> HHAADYVLYKDATKPVEDRVADLLGRMTLAEKIGQMTQIERLVATPDVLRDNFIGSLLSGGGSV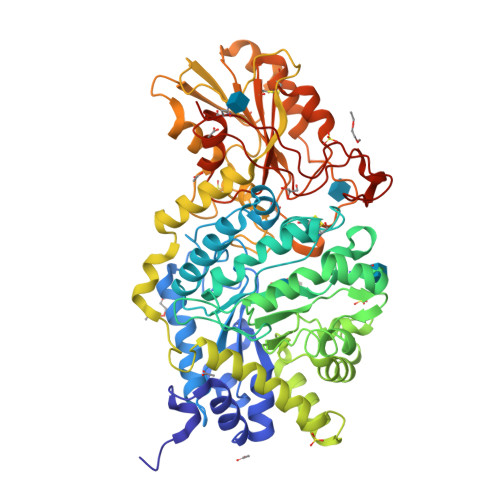PRKGATAKEWQDMVDGFQKACMSTRLGIPMIYGIDAVHGQNNVYGATIFPHNVGLGATRDPYLVKRIGEATALEVRATGIQYAFAPCIAVCRDPRWGRCYESYSEDRRIVQSMTELIPGLQGDVPKDFTSGMPFVAGKNKVAACAKHFVGDGGTVDGINENNTIINREGLMNIHMPAYKNAMDKGVSTVMISYSSWNGVKMHANQDLVTGYLKDTLKFKGFVISDWEGIDRITTPAGSDYSYSVKASILAGLDMIMVPNKYQQFISILTGHVNGGVIPMSRIDDAVTRILRVKFTMGLFENPYADPAMAEQLGKQEHRDLAREAARKSLVLLKNGKTSTDAPLLPLPKKAPKILVAGSHADNLGYQCGGWTIEHQGDTGRTTVGTTILEAVKAAVDPSTVVVFAENPDAEFVKSGGFSYAIVAVGEHPYTETKGDNLNLTIPEPGLSTVQAVCGGVRCATVLISGRPVVVQPLLAASDALVAAWLPGSEGQGVTDALFGDFGFTGRLPRTWFKSVDQLPMNVGDAHYDPLFRLGYGLTTNATKKY>[2x]MLDITTITRQNVTSVVGYYSDAKDDYYSKDSSFTSWQGTGAEALGLSGDVESARFKELLVGEIDTFTHMQRHVGDAKKERL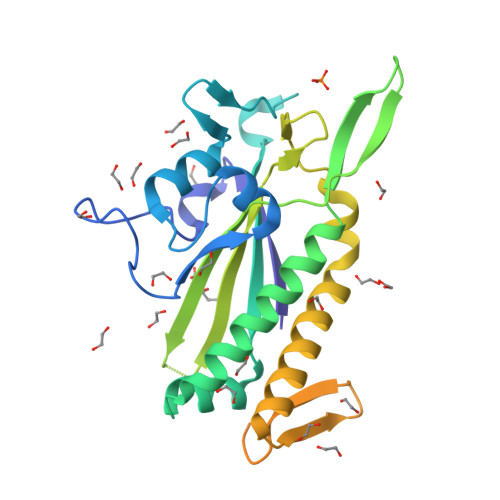GYDLTFSAPKGVSMQALIHGDKTIIEAHEKAVAAAVREAEKLAQARTTRQGKSVTQNTNNLVVATFRHETSRALDPDLHTHAFVMNMTQREDGQWRALKNDELMRNKMHLGDVYKQELALELTKAGYELRYNSKNNTFDMAHFSDEQIRAFSRRSEQIEKGLAAMGLTRETADAQTKSRVSMATREKKTEHSREEIHQEWASRAKTLGIDFDNREWQG>[6x]MGSSHHHHHHSSGLVPRGSGSDPTRKQKVEAQKQAEKLMKQIGVKNVKLSEYEMSIAAHLVDPLNMHVTWSDIAGLDDVITDLKDTVILPIKKKHLFENSRLLQPPKGVLLYGPPGCGKTLIAKATAKEAGCRFINLQPSTLTDKWYGESQKLAAAVFSLAIKLQPSIIFIDQIDSFLRNRSSSDHEATAMMKAQFMSLWDGLDTDHSCQVIVMGATNRPQDLDSAIMRRMPTRFHINQPALKQREAILKLILKNENVDRHVDLLEVAQETDGFSGSDLKEMCRDAALLCVREYVNSTSEESHDEDEIRPVQQQDLHRAIEKMKKSKDAAFQNVLTHVCLD

The mitochondrial AAA (ATPase Associated with diverse cellular Activities) protein ATAD1 (in humans; Msp1 in yeast) removes mislocalized membrane proteins, as well as stuck import substrates from the mitochondrial outer membrane, facilitating their re-insertion into their cognate organelles and maintaining mitochondria’s protein import capacity. ATAD1 is a member of a large family of proteins called the AAA (ATPase Associated with diverse cellular Activities) proteins. Six ATAD1 subunits rotate and translocate progressively to form a hexameric spiral assembly. Each ATAD1 subunit consists of two subdomains, a large subdomain followed by a small subdomain, and the nucleotide is bound at the interface between the two.

To obtain a homogenous sample for structural analysis, we expressed human ATAD1 lacking the first 40 amino acids (consisting of the transmembrane helix) with an N-terminal His-tag and bearing a commonly used ‘Walker B’ mutation that inactivates ATP hydrolysis but retains ATP binding (Δ40-ATAD1E193Q). Δ40-ATAD1E193Q formed oligomers as assessed by size exclusion chromatography. 3D classification of the particles resulted in two distinct hexameric structures. In the second structure, the subunits are arranged in a similar fashion as the first, with the exception of M6, which is in transition to convert into M1 as part of the AAA protein functional ATPase cycle and now bridges M1 and M5, closing the hexameric ring (96,577 particles analyzed). This structure closely resembles the ‘closed state’ structure observed in Msp1. Refinement of this structure yielded a map with an average resolution of 3.2 Å with most of the side chain densities clearly visible, which allowed us to build an atomic model. Noticeably, the density of the M6 subunit in the ‘closed state’ structure was less well defined than the rest of the complex (local resolution ranging from 4 to 6 Å), indicating a mixture of different states. By contrast, for ATAD1, we could identify secondary structure elements clearly, which enabled us to build a polyalanine model for this subunit. To initiate the subunit translocation, the M6 subunit loses its bound nucleotide, and translocates upward to bridge the gap with M1. Meanwhile, the small subdomain of M5 rotates toward its large subdomain, allowing it to establish contacts with the small subdomain of M6 in the ‘closed state’ structure. While examining the interactions of the mobile subunit (M6) in the closed conformation, we noticed that it is held in place by contacts on both sides: on the side of M5, substantial contacts exist between the large and the small subdomains of the two subunits.>MGSSHHHHHHSSGLVPRGSHHEGHAQAPGTHQTRHGGMTTVGEVDHEKNGF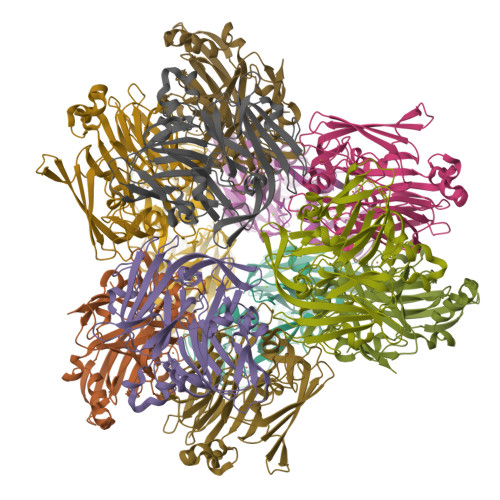DPYAFLTHWETGEVSTLPSGQTLREFNIVAVDKEIEIAPGVYFPAWTYNGQVPGPTLRVTEGDRVRVHFHNAGSHPHTIHFHGIHPASMDGVPGTGPGMIYPGESFTYEFDAYPFGCHLYHCHAIPLKRHIHKGLYGAFIIDPDPERHPEYQAAARARLLGTPENQAWQEFVMVMNGFDTNFDEENEVYAVNTVAHAYMKRPIRIERDRPVRIYLINATEFDPINSFHLHANFFDYYDHGTTLTPTLKTVDTIMQCQGQRGILEFSFNGFEPGLYMFHAHQSEFAELGWMGNFEVIE[8x]To prevent this, we describe a method to encapsulate target proteins within highly hydrophilic, structurally homogeneous, and stable protein shells, which we refer to as “nanocrates” for this purpose. Our approach was inspired by the established use of natural virus capsids and engineered protein containers for packaging applications. We adapted this concept for cryo-EM by encapsulating target proteins within symmetric MS2 bacteriophage-derived “nanocrates”. Being highly symmetric, the nanocrates do not adopt a preferred orientation at the AWI, and therefore their enveloped cargoes are randomly oriented. Nanocrate densities can be computationally subtracted during single-particle cryo-EM analysis to allow for high-resolution reconstruction of the molecules inside.

MS2 virus-like particles have multiple properties that make them ideal for use as nanocrates. They are expressed and isolated in high yields and are amenable to controlled disassembly and reassembly around cargo proteins by a simple pH-dependent protocol. Disassembled MS2 coat proteins can be stored at 4^°^C for at least a day and at -80^°^C for several months without losing reassembly and encapsulation efficiency. Briefly, we purified MS2 capsids from *E. coli*, performed disassembly in an acidic solvent with the removal of packaged viral RNA by centrifugation, and reassembled the capsid proteins at neutral pH in the presence of ApoF.

>ASNFTQFVLVDNGGTGDVTVAPSNFANGVAEWISSNSRSQAYKVTCSVRQSSAQNRKYTIKVEVPKVATQTVGGVELPVAAWRSYLNMELTIPIFATNSDCELIVKAMQGLLKDGNPIPSAIAANSGIY[3x]> RPKLSEEQQHIIAILLDAHHKTYDPTYADFRDFRPPVRMDGSTGSVTLDLSPLSMLPHLADLVSYSIQKVIGFAKMIPGFRDLTSDDQIVLLKSSAIEVIMLRSNQSFTMDDMSWDCGSQDYKYDVTDVSKAGHTLELIEPLIKFQVGLKKLNLHEEEHVLLMAICIVSPDRPGVQDAKLVEAIQDRLSNTLQTYIRCR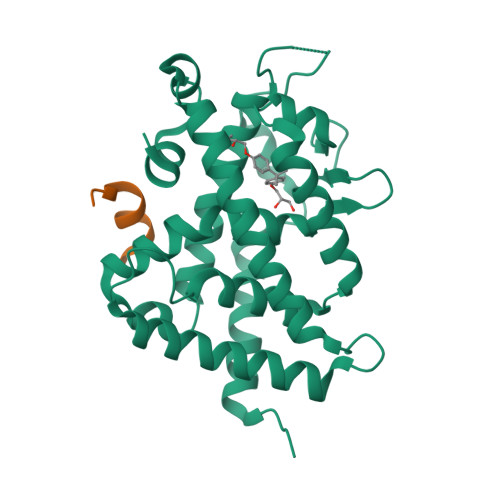HPPPGSHQLYAKMIQKLADLRSLNEEHSKQYRSLSFQPENSMKLTPLVLEVFGN;> KNHPMLMNLLKDN>SNAGKNVMVEPHRHEGVFICRGKEDALVTKNLVPGESVYGEKRVSISEGDDKIEYRAWNPFRSKLAAAILGGVDQIHIKPGAKVLYLGAASGTTVSHVSDIVGPDGLVYAVEFSHRSGRDLINLAKKRTNIIPVIEDARHPHKYRMLIAMVDVIFADVAQPDQTRIVALNAHTFLRNGGHFVISIKANCIDSTASAEAVFASEVKKMQQENMKPQEQLTLEPYERDHAVVVGVYRPPPKVKN[2x]

Fibrillarin (FBL) is an essential and evolutionarily highly conserved S-adenosyl methionine (SAM) dependent methyltransferase. It is the catalytic component of a multiprotein complex that facilitates 2′-O-methylation of ribosomal RNAs (rRNAs), a modification essential for accurate and efficient protein synthesis in eukaryotic cells. Fibrillarin consists of an N-terminal glycine–arginine-rich domain (GAR), which is believed to be important for organisation of the nucleolus, and a C-terminal domain with a Rossmann fold that is characteristic of class I S-adenosylmethionine (SAM)-dependent methyltransferases. In the present study, we determined, to our knowledge, the first crystal structures of hFBL in ligand-free state, bound to the native cofactor SAM, and in complex with two fragments that can compete with SAM for binding to the cofactor site.

We selected 4 derivatives of 1, namely 1a, 1b, 1c, and 1d. They all have an amide linker that connects a synthetically convenient analogue of 1 and an amino acid, the latter of which showed potential to stabilise the loop W137-K143 via ionic interactions between their terminal carboxylate group and the amino moiety on the side chain of K143. A different orientation of the fused bicyclic ring was observed for 1a from 1 with concomitant movements of some binding site residues, especially D236. In addition, electron density for 1a was not observed beyond the amide linker, which appeared to be turning away from the catalytic site and pointing towards the bulk solvent. This indicates that the extended D-phenylalanine moiety did not bind as well as the methionine portion of SAM, and was consequently exposed to the bulk solvent, which in turn affects the orientation of the fused bicyclic ring. Indeed, the binding affinity of 1a turned out to be similar to that of 1. In addition to 1a, 1c, 1d, and a synthetic intermediate without the amino acid 1e were also shown to compete with SAM binding to hFBL in solution by STD NMR assays.> MEGLAGYVYKAASEGKVLTLAALLLNRSESDIRYLLGYVSQQGGQRSTPLIIAARNGHAKVVRLLLEHYRVQTQQTGTVRFDGYVIDGATALWCAAGAGHFEVVKLLVSHGANVNHTTVTNSTPLRAACFDGRLDIVKYLVENNANISIANKYDNTCLMIAAYKGHTDVVRYLLEQRADPNAKAHCGATALHFAAEAGHIDIVKELIKWRAAIVVNGHGMTPLKVAAESCKADVVELLLSHADCDRRSRIEALELLGASFANDRENYDIIKTYHYLYLAMLERFQDGDNILEKEVLPPIHAYGNRTECRNPQELESIRQDRDALHMEGLIVRERILGADNIDVSHPIIYRGAVYADNMEFEQCIKLWLHALHLRQKGNRNTHKDLLRFAQVFSQMIHLNETVKAPDIECVLRCSVLEIEQSMNRVKNISDADVHNAMDNYECNLYTFLYLVCISTKTQCSEEDQCKINKQIYNLIHLDPRTREGFTLLHLAVNSNTPVDDFHTNDVCSFPNALVTKLLLDCGAEVNAVDNEGNSALHIIVQYNRPISDFLTLHSIIISLVEAGAHTDMTNKQNKTPLDKSTTGVSEILLKTQ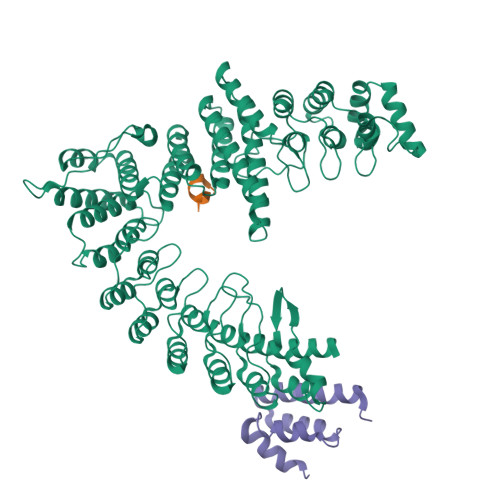MKMSLKCLAARAVRANDINYQDQIPRTLEEFVGFH;> DRKRRSDPNFKNRLRERRKKQKLAKERAGLSKLPDLKDAEAVQKFFLEEIQLGEELLAQGEYEKGVDHLTNAIAVCGQPQQLLQVLQQTLPPPVFQMLLTKLPTISQRIVSAQSLAEDDVE>[14x]MGQAFFKKIVGCFCLGYLFLSSAIEAAALDIKNFNRGRVKVVNKKIAYLGDEKPITIWTSLDNVTVIQLEKDETISYITTGFNKGWSIVPNSNHIFIQPKSVKSNLMFEKEAVNFALMTRDYQEFLKTKKLIVDAPDPKELEEQKKALEKEKEAKEQAQKAQKDKREKRKEERAKNRANLENLTNAMSNPQNLSNNKNLSEFIKQQRENELDQMERLEDMQEQAQANALKQIEELNKKQAEETIKQRAKDKINIKTDKPQKSPEDNSIELSPSDSAWRTNLVVRTNKALYQFILRIAQKDNFASAYLTVKLEYPQRHEVSSVIEEELKKREEAKRQKELIKQENLNTTAYINRVMMASNEQIINKEKIREEKQKIILDQAKALETQYVHNALKRNPVPRNYNYYQAPEKRSKHIMPSEIFDDGTFTYFGFKNITLQPAIFVVQPDGKLSMTDAAIDPNMTNSGLRWYRVNEIAEKFKLIKDKALVTVINKGYGKNPLTKNYNIKNYGELERVIKKLPLVRDK

The H. pylori Cag T4SS is of particular interest because of its role in translocating CagA (a bacterial oncoprotein) into host cells, an important step in gastric cancer pathogenesis. Here we report the use of single particle cryo-EM to determine the structure of a transmembrane Cag T4SS complex extracted and purified from H. pylori. The structure can be divided into three major regions: the OMCC, a periplasmic ring complex (PRC), and a central stalk. The OMCC has a structural organization markedly different from that of T4SS OMCCs in other species, and there is an unexpected symmetry mismatch between the 14-fold-symmetric OMCC and a contiguous 17-fold-symmetric PRC.

The C-terminal portion of CagX is comprised of two β-sheets preceded by a long helix. This helix extends from the top of the O-layer through the central chamber into the I-layer of the OMCC. The C-terminal portion of CagY is structurally similar to VirB10 and TraF homologs, and the C-terminal portion of CagX is structurally similar to VirB9 and TraO homologs. Both CagY and CagX are much larger in size than characterized VirB/Tra homologs, and correspondingly, CagX has a long α-helix that is absent in the structures of TraO or VirB9 (4, 5). Analysis of the 5.4 Å structure suggests that the connection between OMCC and PRC may occur by contacts between the 14 α-helices extending from the N-terminus of CagX and the 17 unidentified α-helices extending up from the PRC. The tips of these α-helices are presumed to be flexible, since the corresponding densities are not well defined in the higher resolution maps.> MTLETTLFPLEGTGACGASYQLYAVKGLSGLDETEYHKNVNLLVRRLSFS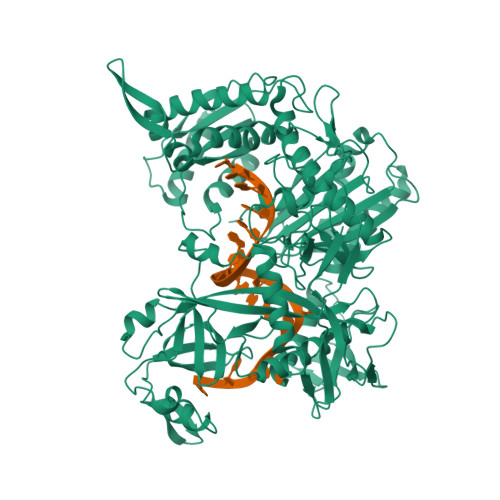MKAPFVALSRDGEQFIAVPNYVTEFPVDHRVVRAMVKLVPTGEPLNLRFDAADDEYDGLRLRYLDFVLQQPLFANHHLWQPGSGQPFFHKKPLKRLDDVDLYDGVSVRAAKHPEGGFGIVCDARSKFITHTPIGARADRKRLGKLINRSCLYKMGDHWYQFRIDAVSDWKVGEPSLFEGNVPISLAQQLVRTAGNAAPKSIIDLDPEGGALEYFTSTNERRMAPAELCFLIEDTHGRRAAKLQRQTILSPSERRARVNGFIRRYLSELNIGGAKLSAGARAHAFFTETHMPPALSFGNGTVLAPDTSKDRFQAMQEYSSMRRTMMLDKKVGFFHQDVFPPQTLLLPESVKKSWGPAFASDFVGTVQELYPAGGYRPEIIEYRDKAYGGGVPGQMKALLEVAERGEIKSGDVLVMLHRINGAPRAQDKLAAMVCNEFEKRFGKRVQVIHSDSPGRGYKRIFKNDKPTYVQQRGRGVNIKGYLKGAALNKVCLGNSRWPFVLRDPLNADVTIGIDVKNNMAVFTMVAEGGRIVRVQRSRSRQREQLLESQVTQVITEMLSKELPEIKKQVQRVVIHRDGRAWPAEIAGARKTFADMAESGLIAVDADVSVFEVLKSSPAPLRLFSFEEPTQENPKGVINPVLGSWLKLSENDGYICTTGAPLLLQGTADPLHVRKAFGPMAIEDALKDVFDLSCLTWPKPDSCMRLPLTIKLCDIALFDDAAEYDVDVVRFADGNTGEASA>[20x]HMGSDEPAQAEASQQVQAKASDASPIAYVNLPQAFVFNVTG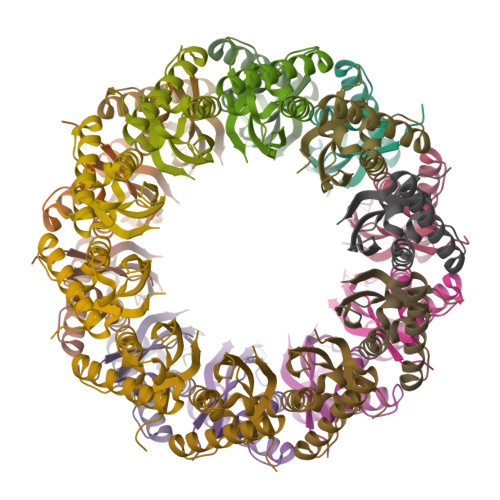DSRDRLVQIKAQLMVRGAENEELARYHSPLIESSLLSTFASATVDQLRSPTGRVELRDRASEDIKAALNAAVGKPVIEKVLFTDFVIQ L-gamma-glutamyl-S-(2-carboxyethyl)-L-cysteinylglycine 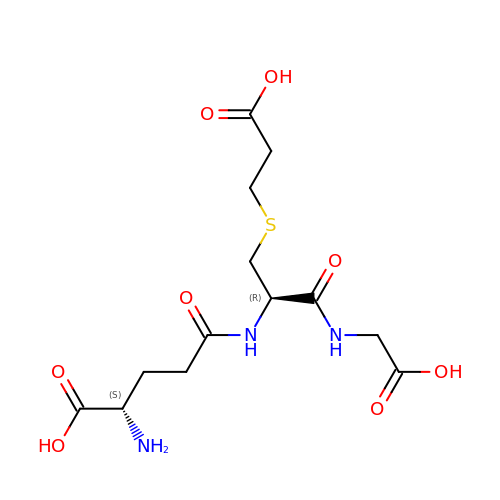| C13 H21 N3 O8 S | ILLXYSCGSHMUFK-YUMQZZPRSA-N> VHATPLIRRLAREF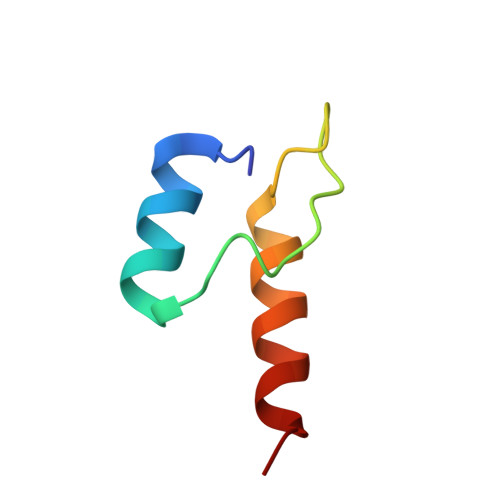GVNLAKVKGTGRKGRILREDVQAYVKEAIKRA>[5x]IEKQMDRVVKEMRRQLEMIDK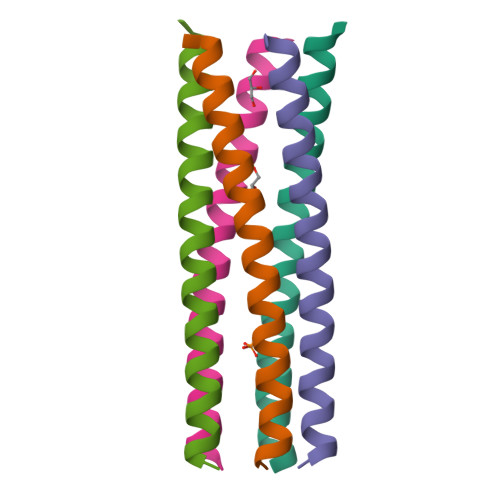LTTRAIEAVELLKRIYDKLTVQTTGEIDMTK The L-arginine biosynthesis pathway consists of eight enzymes that catalyse the conversion of L-glutamate to L-arginine, appears to be attractive target for anti-Tuberculosis (TB) drug discovery. The arginine biosynthesis pathway consists of eight different enzymes ([Fig fig1]) all considered to be essential for *M. tuberculosis* growth *in vitro*. In this work, the ligandability of four enzymes of the pathway ArgB, ArgC, ArgD and ArgF is explored using a fragment-based approach. In conclusion, using a fragment-based approach, we have discovered inhibitors that bind to novel sites in ArgB and ArgF and to the active sites of ArgC and ArgD, which in case of ArgB show on target activity against *M. tuberculosis*.

Additionally, structures were solved with 4 fragment binders, occupying either of the two distinct pockets: the substrate-binding ([Fig fig2] and [Fig fig2]) and the NADP(H)-binding pockets ([Fig fig2] and [Fig fig2]). 2 mM NMR401 inhibited ArgC activity by 10% whereas 2 mM NMR863 caused a 12% inhibition. Although the thermal shifts obtained for NADP(H)-binding pocket fragments NMR401 and NMR863 were higher than those for substrate-binding pocket fragments NMR322 and NMR571, the SPR binding response for the latter was better and positively correlated with percentage inhibition of enzymatic activity (**[Table tbl2]**). Our results further show that in the case of ArgC there are two possible strategies to develop inhibitors, with one targeting the cofactor binding site and the other the substrate binding site. It is not clear at this point which strategy has the highest potential to result in potent inhibitors.

>GSMQNRQVANATKVAVAGASGYAGGEILRLLLGHPAYADGRLRIGALTAATSAGSTLGEHHPHLTPLAHRVVEPTEAAVLGGHDAVFLALPHGHSAVLAQQLSPETLIIDCGADFRLTDAAVWERFYGSSHAGSWPYGLPELPGARDQLRGTRRIAVPGCYPTAALLALFPALAADLIEPAVTVVAVSGTSGAGRAATTDLLGAEVIGSARAYNIAGVHRHTPEIAQGLRAVTDRDVSVSFTPVLIPASRGILATCTARTRSPLSQLRAAYEKAYHAEPFIYLMPEGQLPRTGAVIGSNAAHIAVAVDEDAQTFVAIAAIDNLVKGTAGAAVQSMNLALGWPETDGLSVVGVAP[8x]> TPAATGKPPALSKGLRSQSSDYTGHVHPGTYTNTLERLVKEMEDTQRLDELQKQLQEDIRQGRGIKSPIRIGEEDSTDDEDGLLEEHKEFLKKFSVTIDAIPDHHPGEEIFNFLNSGKIFNQYTLDLRDSGFIGQSAVE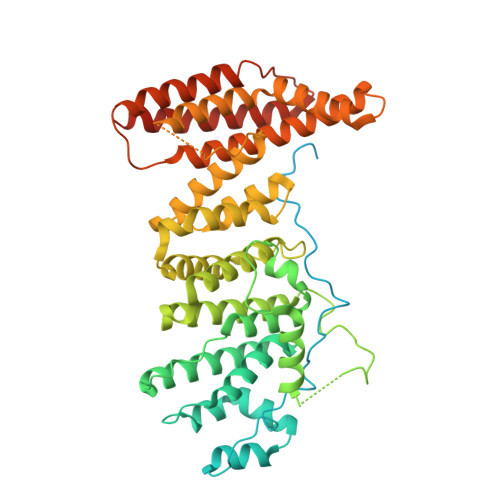KLILKSGKTDQIFLTTQGFLTSAYHYVQCPVPVLKWLFRMMSVHTDCIVSVQILSTLMEITIRNDTFSDSPVWPWIPSLSDVAAVFFNMGIDFRSLFPLENLQPDFNEDYLVSETQTTSRGKESEDSSYKPIFSTLPETNILNVVKFLGLCTSIHPEGYQDREIMLLILMLFKMSLEKQLKQIPLVDFQSLLINLMKNIRDWNTKVPELCLGINELSSHPHNLLWLVQLVPNWTSRGRQLRQCLSLVIISKLLDEKHEDVPNASNLQVSVLHRYLVQMKPSDLLKKMVLKKKAEQPDGIIDDSLHLELEKQAYYLTYILLHLVGEVSCSHSFSSGQRKHFVLLCGALEKHVKCDIREDARLFYRTKVKDLVARIHGKWQEIIQNCRPTQGQLHDFWVPDS>EDICFIAGIGDTNGYGWGIAKELSKRNVKIIFGIWPPVYNIFMKNYKNGKFDNDMIIDKDKKMNILDMLPFDASFDTANDIDEE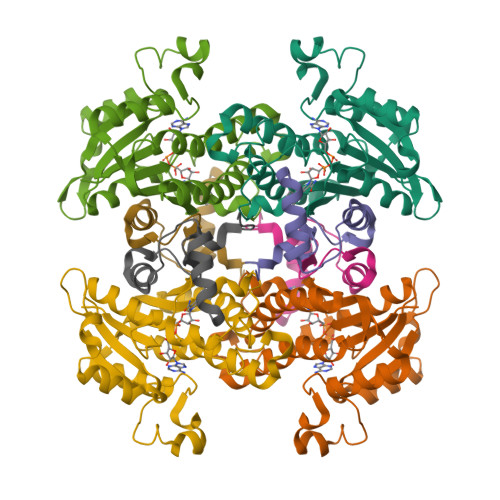TKNNKRYNMLQNYTIEDVANLIHQKYGKINMLVHSLANAKEVQKDLLNTSRKGYLDALSKSSYSLISLCKYFVNIMKPQSSIISLTYHASQKVVPGYGGGMSSAKAALESDTRVLAYHLGRNYNIRINTISAGPLKSRAATAINK[2x];>[2x]YTFIDYAIEYSEKYAPLRQKLLSTDIGSVASFLLSRESRAITGQTIYVDNGLNIMFLPDD> MIKPVGSDELKPLFVYDPEEHHKLSHEAESLPSVVISSQAAGNAVMMGAGYFSPLQGFMNVADAMGAAEKMTLSDGSFFPVPVLCLLENTDAIGDAKRIALRDPNVEGNPVLAVMDIEAIEEVSDEQMAVMTDKVYRTTDMDHIGVKTFNSQGRVAVSGPIQVLNFSYFQADFPDTF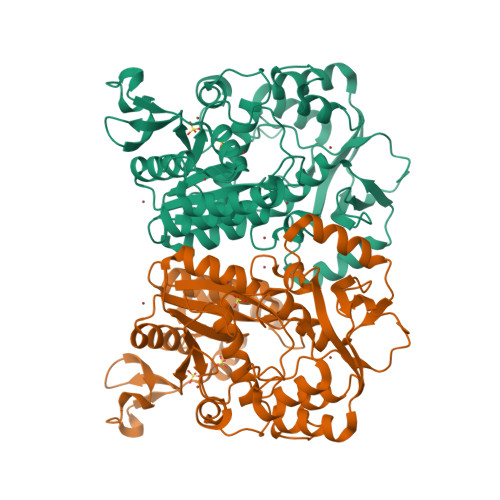RTAVEIRNEIKEHGWSKVVAFQTRNPMHRAHEELCRMAMESLDADGVVVHMLLGKLKKGDIPAPVRDAAIRTMAEVYFPPNTVMVTGYGFDMLYAGPREAVLHAYFRQNMGATHFIIGRDHAGVGDYYGAFDAQTIFDDEVPEGAMEIEIFRADHTAYSKKLNKIVMMRDVPDHTKEDFVLLSGTKVREMLGQGIAPPPEFSRPEVAKILMDYYQSINS>[6x]SNAYTVEPVQDGERSVTLRRAGGTPLVAAMYHLPAAGSPDFVGLDLAATILADTPSSRLYHALVPTKLASG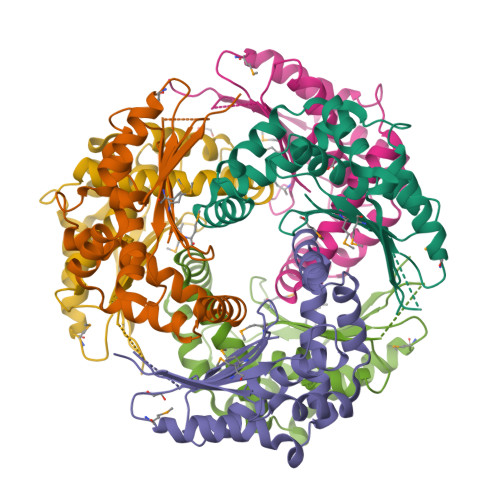VFGFTMDQLDPGLAMFGAQLQPGMDQDKALQTLTATLESLSSKPFSQEELERARSKWLTAWQQTYADPEKVGVALSEAIASGDWRLFFLQRDRVREAKLDDVQRAAVAYLVRSNRTEGRYIPTEKP>MAMSFIKPIYQDINSILIGQKVKRPKSGTLSGHAAGEPFEKLVYKFLKENLSDLTFKQYEYLNDLFMKNPAIIGHEARYKLFNSPTLLFLLSRGKAATENWSIENLFEEKQNDTADILLVKDQFYELLDVKTRNISKSAQAPAIISAYKLAQTCAKMIDNKEFDLF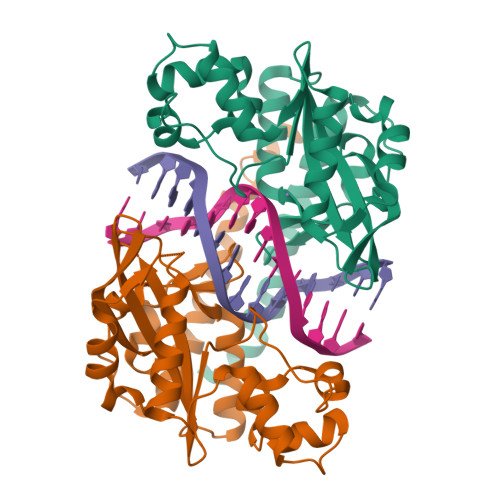DINYLEVDWELNGEDLVCVSTSFAELFKSEPSELYINWAAAMQIQFHVRDLDQGFNGTREEWAKSYLKHFVTQAEQRAISMIDKFVKPFKKYILRSRELVDPNSVQARLQDVDGTIDTRSKLAAAQLYTRASQPELAPEDPEDLEHHHHHH[2x]>[4x]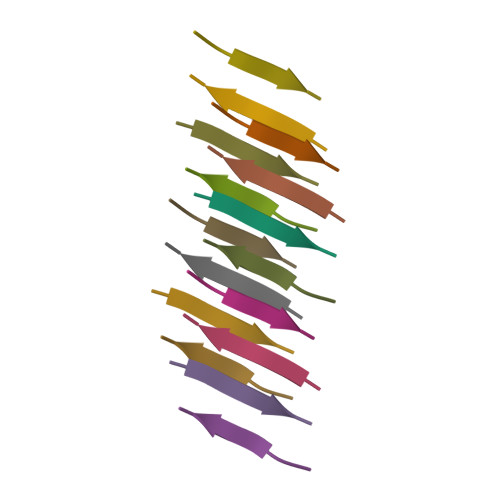NFVFGT> GSHMEAVQNRIVEAAERVPGVRGVIHLRARYVGQDIWADMIIGVDPENTVEQAHEICEAVQAAVCGKIRRIESLHVSAHAREIGDTTKPSFSDQPLSFDE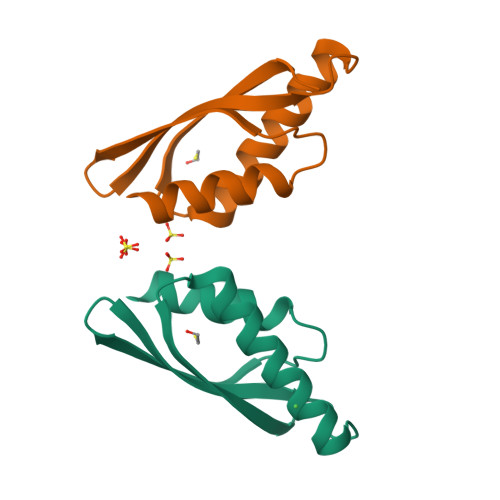VMLSKVDN> MDKNHNTKKILFKNRFVILGFGCVGQALMPLIFEKFDIKPSQVTIIAAEGTKVDVAQQYGVSFKLQQITPQNYLEVIGSTLEENDFLIDVSIGISSLALIILCNQKGALYINAATEPWKEEFVMEKMALNRRTNYSLREEVLRLKDKTQKTALITHGANPGLVSHFIKEALLNIAKDNGLTINRPKNAAEWANLAMTLGIKVIHVAEQDSQVTYPPKSPGEFVNTWSANGLILEGLQPAEIGWGTHEAHWPHDAYSHSNGPQCAIYLSRPSAGVMVRSWTPTLGAFHGFLITHAETISLTNFLTLKNGSELLYRPTVHYAYNPCPDARLSIFELKSN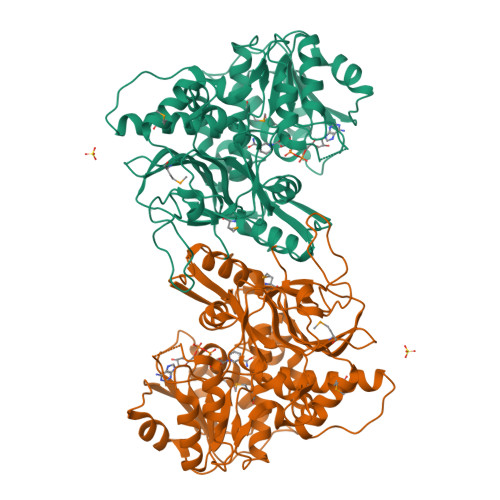EWKPQNKNRLILNEIIDGCDELGVLLMGNQRGAYWYGSTLSIQEARQIAPYNNATSLQVVASMISGIIWAIEHPDEGIVEPEEVDHQYIIDIAKPYLGKVGGYYTDWTPLKNRGELYPEEVDLSDPWQFFNIRVNLEHHHHHH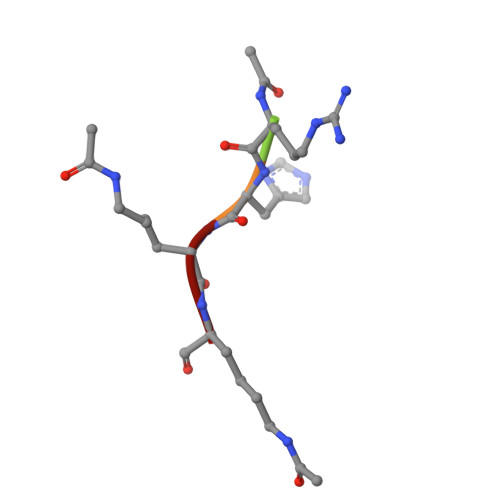> XRHKK>[2x]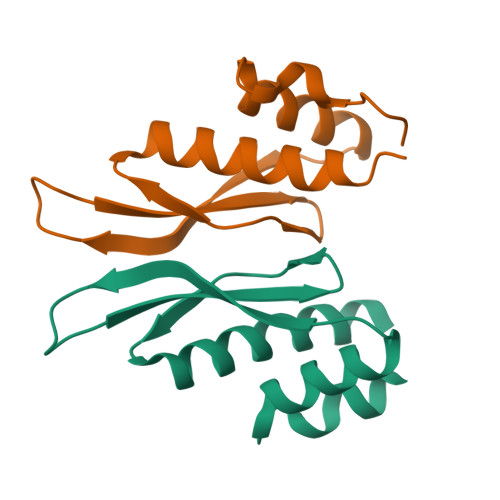GGSAIGELVRYLNTNPVGGLLEYARSHGFAAEFKLVDQSGPPHEPKFVYQAKVGGRWFPAVCAHSKKQGKQEAADAALRVLIGENE>MLVSVYLALLVACVGQAHSQANLMRLKSDLFNRSPMYPGPTKDDPLTVTLGFFLQDIVKVDSSTNEVDLVYYERQRWKLNSLMWDPNEYGNITDFRTSAADIWTPDITAASSTRPVQVLSPQIAVVTHDGSVMFSPAQRLSFMCDPTGVDSEEGVTCAVKFGSFVYSGFEIDLKTDTDQVDLSSYYA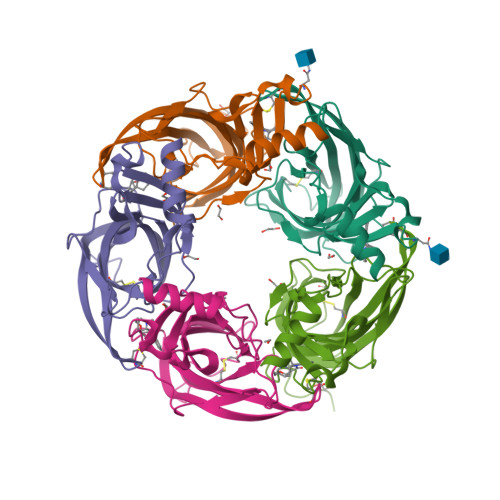SSKYEILSATQTRQVQHYSCCPEPYIDVNLVVKFRERRAGNGFFRNLFDENLYFQGHHHHHH[5x]>[4x]MAPVLENRRARHDYEILETYEAGIALKGTEVKSLRAGKVDF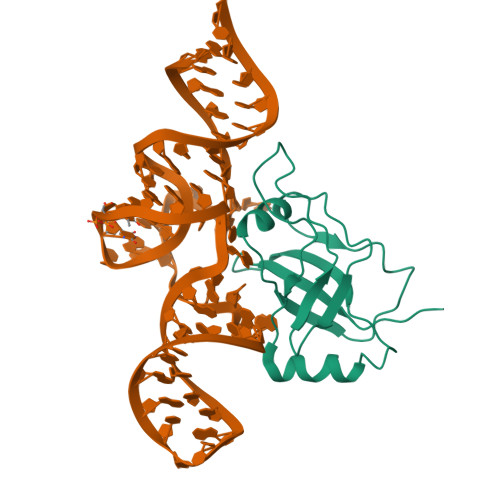TGSFARFEDGELYLENLYIAPYEKGSYANVDPRRKRKLLLHKHELRRLLGKVEQKGLTLVPLKIYFNERGYAKVLLGLARGK>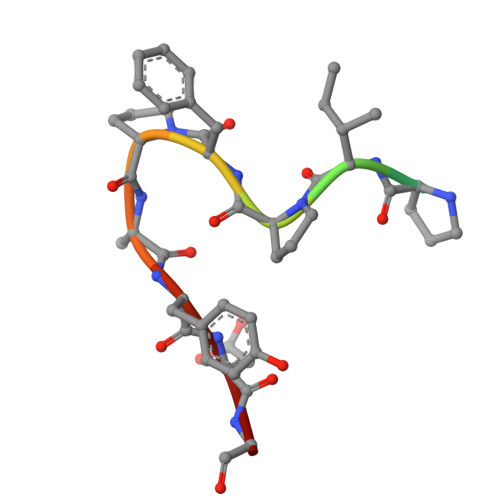 VGAPIPFPAYDG> MSLPKPEDVLVAPNFGIQIDGVMVEYLNSVSNLQIEQDVIRYQQNQGTTGRNNVTLMPGVAKDGSVQVERGMSQSSVFTQWINDSMAGRMATARKNATIIVMDYEDNPVKRWNLRNAWCSKVVAGTLKAGDTNALTETITIVFEELV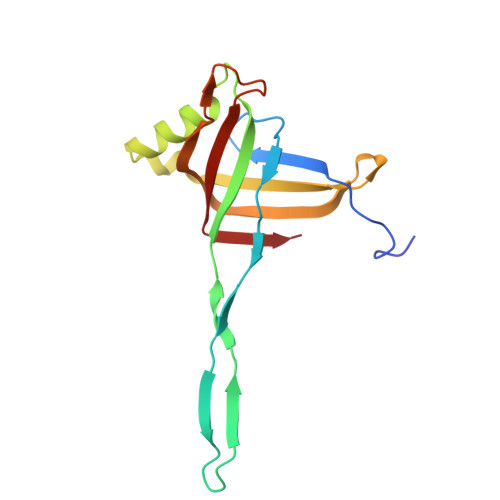VE> M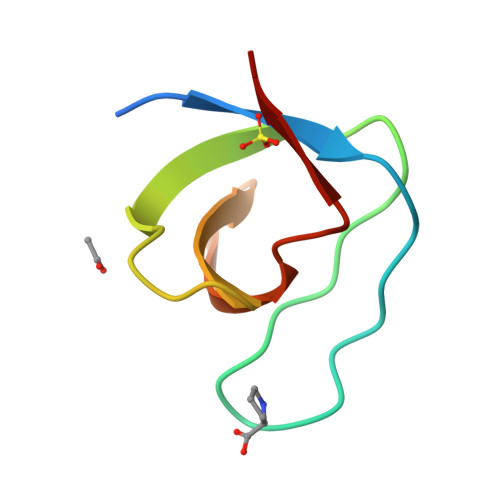DETGKELVLALYDYQEKSPREVTMKKGDILTLLNSTNKDWWKVEVADRQGFVPAAYVKKLD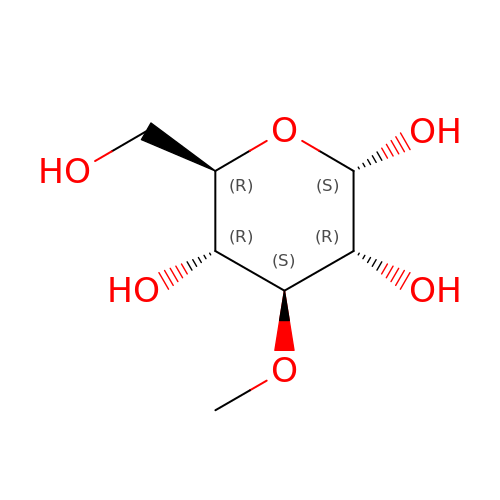3-O-methyl-alpha-D-glucopyranose | C7 H14 O6 | SCBBSJMAPKXHAH-OVHBTUCOSA-N>[2x]GIKGIYKEIGSGERISLCKLAIDHLEQHNRPLRLAIDMAIWQFQIQAARGGSNPAIRTLFYRFVRLLSLGIHPIFVFDGPNKPIFKRNRRSGTGNGVSTAMAKRLIRLFGFTAHDAPGEAEAECAYLEQQGIVDAVLSEDVDTIMFGSRVTLRDWSSEGSKGGPPTHVTLHDAKKIAEGPSGLDREGMVLVALMSGGDYLPDGIPGCGIKVACQAAKAGFGKELCRIKRADKEAITEWKQRLLHELRTNESGFFRTKHKALEIPENFPNMEVLRYYTHPVVSSPATIERLRQEFPPSSTVDIAGLREFTRETFDWTFRPGAIKLIKVLAPGLLVQRCLDRYVSGPRIDDPDLKKKEESTLVKGISMRREHFSTDATPELRVSFIPAELVGLDPGQEPEVQVEAFGRSGLALNSDDEFDEDISSSQKAPKKPFDPWQPDLAWVPETILKLGVPVTVEDWEEGQRS

GEN1 is a member of a superfamily of structure-selective nucleases (Grasby et al., 2012). The structure of the GEN1 protein reveals it to have an elaborated FEN-XPG family fold that is modified for its role in four-way junction resolution. In free solution the protein exists primarily in monomeric form, but binds to DNA junctions as a discrete dimer to generate bilateral cleavage by accelerating second strand cleavage. We have now solved a crystal structure of active GEN1 from C. thermophilum bound to the DNA resulting as the product of cleavage.

In our experiments, we crystallized a wild-type sequence in the presence of Mg2+ ions. Under these conditions, CtGEN1 is fully active, and the species crystallized is the product of resolution cleavage. The presence of MgCl2 in the crystallization solution induced cleavage of the four-way DNA junction by CtGEN1. Electrophoretic analysis of the DNA contents of our crystals shows that the crystallization has selected one of the two products, i.e., that with the intact r strand. The crystallization process has selected a single product of enzymatic cleavage, containing the 30 nt r strand from the junction and the 3′ half of the h strand and the 5′ half of the x strand, i.e., the product with R and X arms. The functional unit is thus one CtGEN1 monomer with one complete DNA product. We have, therefore, associated the 30 nt strand as one covalently continuous strand within the complex and will represent it in that manner hereafter. Thus the functional unit contains a product of resolution, comprising a 30 nt r strand, the 14 nt 3′ section of the h strand (referred to subsequently as 3′h) and the 16 nt 5′ section of the x strand (5′x) of which the first and last nucleotides are not visible in the electron density. The 5′ end of the 14 nt strand is located in the active site of the enzyme, indicated by the presence of a bound Mg2+ ion. For the original Mg2+ crystals, a single bound ion (M2) was observed, but after soaking the crystals with MnCl2, two bound metal ions were observed.>[3x]GMSRSPF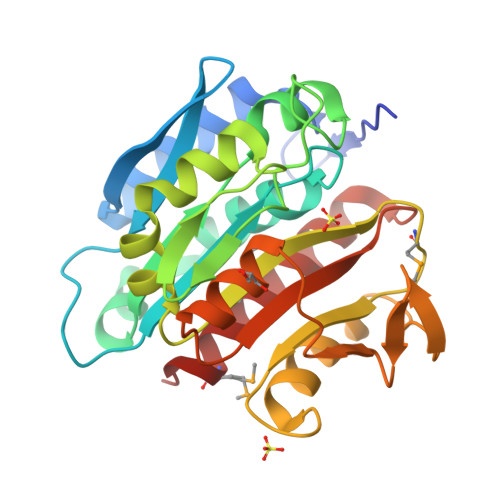QTFVWRSEIFECQSTDIQRFYSLLAIETERLGLGSKILGQAGHHPLYLLQSPGQKAGLPNLLISAGFHGEESAGPWGLLHFLSQLDGELFKRVNLSVLPLVNPTGFAKGHRFNELGENPNRGFFIENGKAKPGADTSAEGRILLEHAHLLQVASRDGILTCHEDVLMTDTYVYTFEPSQAPGRFSHSLRDALGQYFPIAADGDVDNCPVRSGVIFNHFDTSFESFLVRSGARVGCCSETPGQQPLDQRILANAAAMNTFVNMLAPELS> SMLPSYDFFIHPMNLVELKKDIWSDSPVPAKLTYGKKKYDIDIVYRGAHIREFEKKSYHVMFYKPKKFQGAKEFHLNSEFMDPSLIRNKLSLDFFHDIGVLSPKSQHVFIKINGQIQGVYLQLESVDENFLKNRGLPSGSIYYAIDDDANFSLMSERDKDVKTELFAGYEFKYSNENSEEQLSEFVFQANALSREAYEKEIGKFLHVDKYLRWLAGVIFTQNFDGFVHNYALYHNDETNLFEVIPWDYDATWGRDVQGRPLNHEYIRIQGYNTLSARLL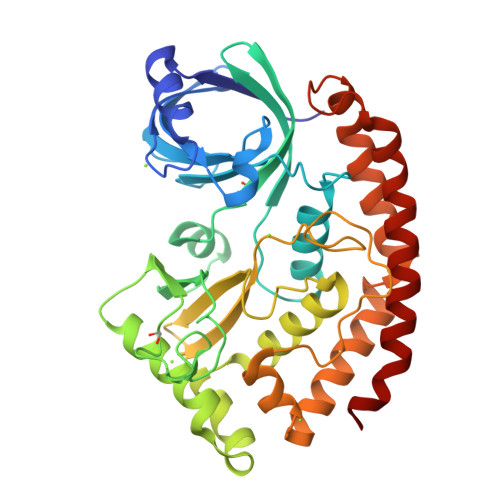DIPIFRKQYRSILEEILAEQFTVSFMMPKVESLCESIRPYLLQDPYMKEKLETFDQEADMIEEYINKRRKYIQDHLHELD Rosellinia necatrix megabirnavirus 1-W779 (RnMBV1) is a non-enveloped icosahedral double-stranded (ds)RNA virus that infects the ascomycete fungus Rosellinia necatrix, a causative agent that induces a lethal plant disease white root rot. RnMBV1 is a potential viro-control approach agent for restraining and controlling the white root rot disease, because the virus can confer hypovirulence to its host fungus. RnMBV1 is an approximately 52 nm bipartite dsRNA mycovirus composed of dsRNA-1 (8.9 kbp in length, AB512282) and dsRNA-2 (7.2 kbp in length, AB512283). The RnMBV1 capsid is composed of 120 chemically identical MCP subunits and additional surface CrPs.

In addition, the 3D reconstruction of the CrPs was obtained by symmetry expansion with 244,609 particle orientations and imposed with C1 symmetry, which generated the final map at 3.3 Å resolution. Small-surface trimeric CrPs are present on the RnMBV1 MCPs at the 3-fold axes. The CrP is composed of C-terminal 135 residues (Lys1292–Gln1426) of the ORF3 in the genome segment dsRNA-2. In addition, each CrP displays α-helix-rich structures, which are formed of seven α-helices (HA–HG). The total interface area between each CrP trimer and three MCP_B subunits at the 3-fold axis is 2.6 x 103 Å2. The interactions are intervened by the hydrophobic interaction of the MCP_B loop Pro548-Lys555 and the CrPs and by one hydrogen bond between MCP_B Arg533 and CrP Gly1341. The CrPs are not present at all 3-fold axes. After 3D focused classification, one CrP trimer was recovered with highest intensity and was deemed to have 100% occupancy, whereas other CrP trimers were 30% occupancy. The averaged CrP trimer numbers per particle are 6.7 for full particles and 8.0 for empty particles, respectively. These results probably reflect their limited and weak interactions with MCPs.

>[3x]MGITYRDAQIFSACVEALSARNNRITLTSFPLTAGQGQAPTATPAWYPVDLFVADATAVYGRRQLFAWTVDKVRPTRNVAFVTDRVAMDFSAALLSLMAELEAVAPDVYAAIHGGATPGADLGDRITQLENRRVGCLAYVMATVVRAPITHNVRSFSAMLASDPQAHAALLAYLTPNSAGQLDGAPIYFRRSDVDLRNNHLALHAEVVPGLPNMVPLTKAMVEVALANVEWWSDPLGYDSLTSFGGLELLSLCDALAVCELSVAYGLKESGYCYLRFAGGCPLAEVILARLGYNPPLGVAVGWALYNGIKLDWYSKVISVGHNMRLHVCDTAGEANACLIDVLTGEYDGMPVGGVDTVSCWVEQLDLLAAAAGVGRNLSNLHCGVQTPPRTINTTRRRLLASLVRTLIADPTLTDEELLHGAVRGTLNGLPRDRALWRCLQVVNTTVREFLAQDLDAMVRDRRECTTYASRAAFAERCAMSGNASGLVGRQYSDMPAALEGEARACGLSAIDAIEIVRVVASGEPIRVLLDQHGRPATRPNGRLTADELRRCRPLVVGQGGQVGFLPFVPFIVGGVGATVAAASGLALATFATVTGAGAVALGGLGLGAGVAALSITVGQLSYQVTRRALTTILPGGREFGLDDLTRVLGGMVGRYISFVDTWFAHGRGDVFQETDAVPAGTVVFVLPNIEYEVLELRERALGRWSTLLVTTPNGVIAMRANGALPLRVVDAREAGQTFEWSTAARRRFTRAQANAINMMVTASKRVPGLKGSIDAAPSQGTGGSGTDLAGILQRLSALEQTSVPRAEFDALQGRVAACEAKITELEADRVPRIDFTELRDRVHHIDGIGLSCLAHLARDLGITVPHNVRTFRQMRANVGEVIWARFVDAVAESFSPMGGRPIFVRTDPAQPRNNHVSLVDEPTTTGFNGTVTPAMRRLTVADLTGDLVDTEWFSWTPYDASGPLGGTIEGIEAYLTDFTSKLKAELEATPTRTELGVAVGTRAPPLSDRLAAVERVIGMQEGNQVWRSNELRELWVAIDSIVTGRGQREFTTATIKWPAAFPSAVATAGRSFGQPGLAGYGELCTLARQLNALVAGVRNGVVSGMTRNGAGVLQLSTISSATGNLTSDQQAVLRACFFPATPRVGEYQIVYPVGGTMGLTRVDPSTNSSIGQYTRESLVAARNAMPRFAVHTTTPDTVGVAWDNQSAAGLPMGAAPVLTVSVNQLSGVPVTEADKQRWDAKQDKFKIVNTDDRVAALSWVDSVDGFAAPGSDMLLDYQAPAGTGSLPFGSKYAMAVAIGGSLGSQLSEAQVSAARVVLGNGVWRDAVIDVLRKLHNVMYGGKYGRIDDIAAMRSYLNDGTGLLPGSEPIVDVGGAEGNACARATILLRGFSSTMVGVDLKIQMLVELYGAEPATAALLYRGWTMQ>[2x]AAPDEITTAWPVN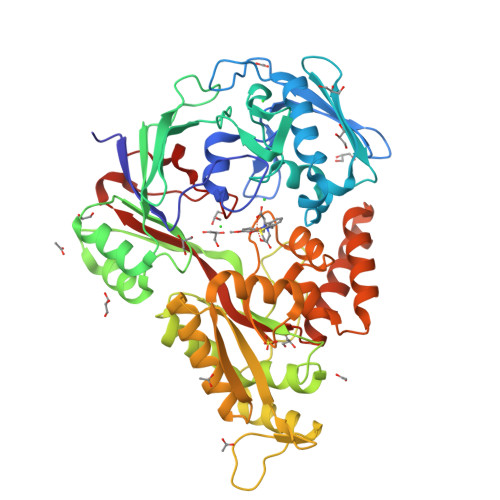VGPLNPHLYTPNQMFAQSMVYEPLVKYQADGSVIPWLAKSWTHSEDGKTWTFTLRDDVKFSNGEPFDAEAAAENFRAVLDNRQRHAWLELANQIVDVKALSKTELQITLKSAYYPFLQELALPRPFRFIAPSQFKNHETMNGIKAPIGTGPWILQESKLNQYDVFVRNENYWGEKPAIKKITFNVIPDPTTRAVAFETGDIDLLYGNEGLLPLDTFARFSQNPAYHTQLSQPIETVMLALNTAKAPTNELAVREALNYAVNKKSLIDNALYGTQQVADTLFAPSVPYANLGLKPSQYDPQKAKALLEKAGWTLPAGKDIREKNGQPLRIELSFIGTDALSKSMAEIIQADMRQIGADVSLIGEEESSIYARQRDGRFGMIFHRTWGAPYDPHAFLSSMRVPSHADFQAQQGLADKPLIDKEIGEVLATHDETQRQALYRDILTRLHDEAVYLPISYISMMVVSKPELGNIPYAPIATEIPFEQIKPVKP>[2x]MENFPTEYFLNTTVRLLEYIRYRDSNYTREERIENLHYAYNKAAHHFAQPRQQQLLKVDPKRLQASLQTIVGM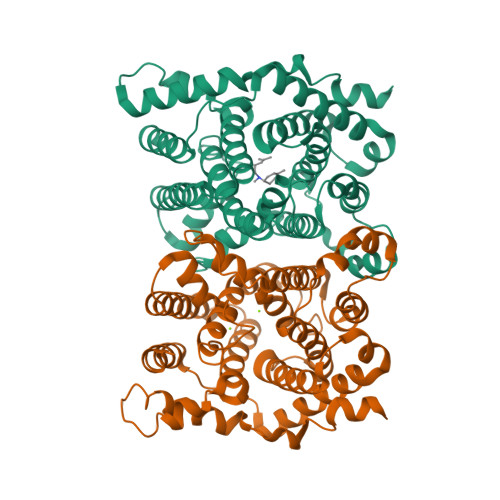VVYSWAKVSKECMADLSIHYTYTLVLDDSKDDPYPTMVNYFDDLQAGREQAHPWWALVNEHFPNVLRHFGPFCSLNLIRSTLDFFEGCWIEQYNFGGFPGSHDYPQFLRRMNGLGHCVGASLWPKEQFNERSLFLEITSAIAQMENWMVWVNDLMSFYKEFDDERDQISLVKNYVVSDEISLHEALEKLTQDTLHSSKQMVAVFSDKDPQVMDTIECFMHGYVTWHLCDRRFRLSEIYEKVKEEKTEDAQKFCKFYEQAANVGAVSPSEWAYPPVAQLANVRSKDVKEVQKPFLSSIELVE1-[5-chloro-4-({6-chloro-7-[1-(oxetan-3-yl)piperidin-4-yl]quinazolin-2-yl}amino)-1H-pyrazol-1-yl]-2-methylpropan-2-ol 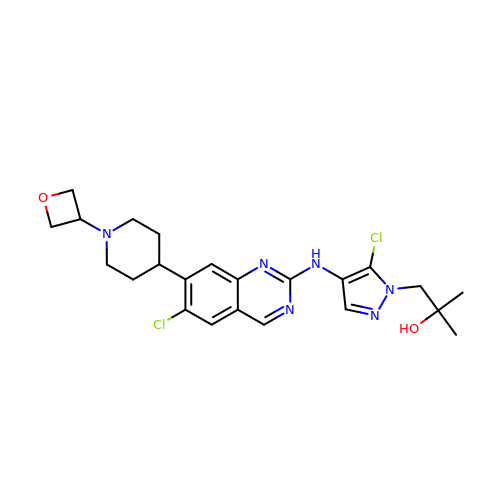| C23 H28 Cl2 N6 O2 | MYRFCAOJVUFSNI-UHFFFAOYSA-N>[4x]ETMKFMAENRLTLTKGTAKDIIERFYTRHGIETLEGFDGMFVTQTLE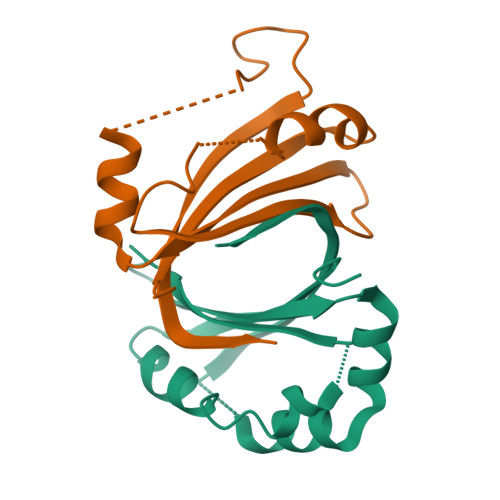QEDFDEVKILTVWKSKQAFTDWLKSDVFKAAHKHVRSKNEDESSPIINNKVITYDIGYSYMK>[2x]MKSVVTTVLAAADAAGRFPSGSDLESVQGNIQRSAARL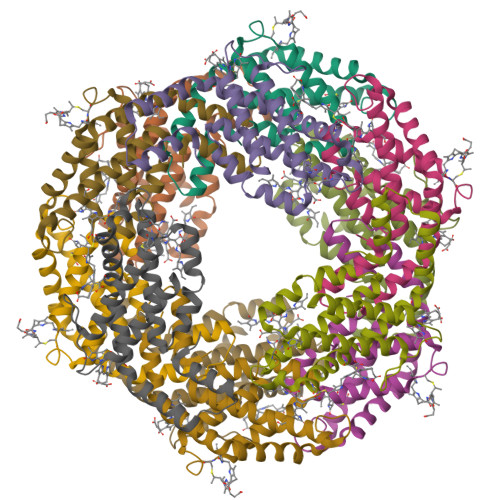EAAEKLAAGHAAVVKEAGDVVFKKYPYLKTAGEAGDSAEKVAKCYRDIDHYMRLINYCLVVGGTGPLDEWGISGAREVYRALNLPTAAYVAAFQYTRDRACAPRDMGPQALTEFRSYLDYVINALS;>MLDAFSKAVVSADQKTGYIGGAELAALKTYIANGNKRLDAVNAITSNASCIVSDAVSGMICENPGLISAGGNCYTNRRMAACLRDGEIVLRYVTYALLAGDASVLEDRCLNGLKETYMALGVPIPSAIRAVSIMKASAVAFINNTASKRKIETPQGDCAALASEAGSYFDMAASALR[2x]> GIEDLIDTAIKNALRVSQPPSTQSTEATSGVNSQEVPALTAVETGASGQAIPSDVVETRHVVNYKTRSESCLESFFGRAACVTILSLTNSSKSGEEKKHFNIWNITYTDTVQLRRKLEFFTYSRFDLEMTFVFTENYPSTASGEVRNQVYQIMYIPPGAPRPSSWDDYTWQSSSNPSIFYMYGNAPPRMSIPYVGIANAYSHFYDGFARVPLEGENTDAGDTFYGLVSINDFGVLAVRAVNRSNPHTIHTSVRVYMKPKHIRCWCPRPPRAVLYRGEGVDMISSAI;> SPNVEACGYSDRVRQITLGNSTITTQEAANAIVAYGEWPTYINDSEANPVDAPTEPDVSSNRFYTLESVSWKTTSRGWWWKLPDCLKDMGMFGQNMYYHYLGRSGYTIHVQCNASKFHQGALGVFLIPEFVMACNTESKTSYVSYINANPGERGGEFTNTYNPSNTDASEGRKFAALDYLLGSGVLAGNAFVYPHQIINLRTNNSATIVVPYVNSLVIDCMAKHNNWGIVILPLAPLAFAATSSPQVPITVT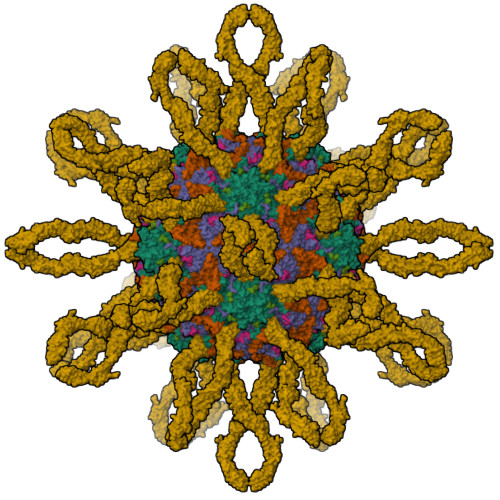IAPMCTEFNGLRNITVPVHQ;> GLPTMNTPGSNQFLTSDDFQSPCALPNFDVTPPIHIPGEVKNMMELAEIDTLIPMNAVDGKVNTMEMYQIPLNDNLSKAPIFCLSLSPASDKRLSHTMLGEILNYYTHWTGSIRFTFLFCGSMMATGKLLLSYSPPGAKPPTNRKDAMLGTHIIWDLGLQSSCSMVAPWISNTVYRRCARDDFTEGGFITCFYQTRIVVPASTPTSMFMLGFVSACPDFSVRLLKDTPHISQSK;> LPLTKVDSITTF;> LIGRTQ;> QTSVSPSKVILPRGGSVLVTCSTSCDQPMLLGIETPLPKKELLLPGNNRKVYELSNVQEDSQPMCYSNCPDGQSTAKTFLTVYWTPERVELAPLPSWQPVGKNLTLRCQVEGGAPRANLTVVLLRGEKELKREPAVGEPAEVTTTVLVRRDHHGANFSCRTELDLRPQGLELFENTSAPYQLQTFVLPATPPQLVSPRVLEVDTQGTVVCSLDGLFPVSEAQVHLALGDQRLNPTVTYGNDSFSAKASVSVTAEDEGTQRLTCAVILGNQSQETLQTVTIYSFPAPNVILTKPEVSEGTEVTVKCEAHPRAKVTLNGVPAQPLGPRAQLLLKATPEDNGRSFSCSATLEVAGQLIHKNQTRELRVLYGPRLDERDCPGNWTWPENSQQTPMCQAWGNPLPELKCLKDGTFPLPIGESVTVTRDLEGTYLCRARSTQGEVTREVTVNVLSP>XFSPAAP[28x];>GHMSFDNYLVPTVIEQSGRGERAFDIYSRLLKERIVFLVGPVTDESANLVVAQLLFLESENPDKDIFFYINSPGGSVTAGMSIYDTMNFIKPDVSTLCLGQAASMGAFLLSAGEKGK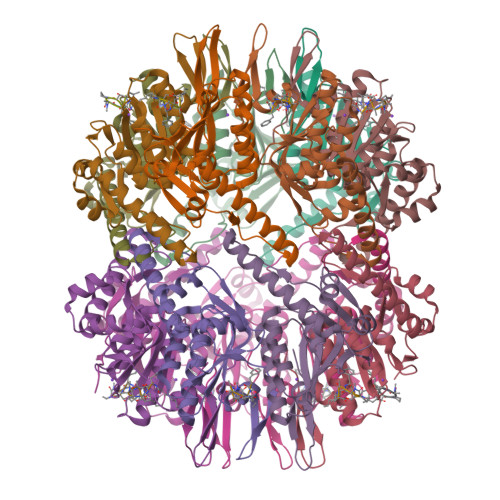RFALPNSRIMIHQPLISGGLGGQASDIEIHARELLKIKEKLNRLMAKHCDRDLADLERDTDRDNFMSAEEAKEYGLIDQILENRASLRL[28x]> MSDTWSSIQAHKKQLDSLRERLQRRRKQDSGHLDLRNPEAALSPTFRSDSPVPTAPTSGGPKPSTASAVPELATDPELEKKLLHHLSDLALTLPTDAVSICLAISTPDAPATQDGVESLLQKFAAQELIEVKRGLLQDDAHPTLVTYADHSKLSAMMGAVAEKKGPGEVAGTVTGQKRRAEQDSTTVAAFASSLVSGLNSSASEPAKEPAKKSRKHAASDVDLEIESLLNQQSTKEQQSKKVSQEILELLNTTTAKEQSIVEKFRSRGRAQVQEFCDYGTKEECMKASDADRPCRKLHFRRIINKHTDESLGDCSFLNTCFHMDTCKYVHYEI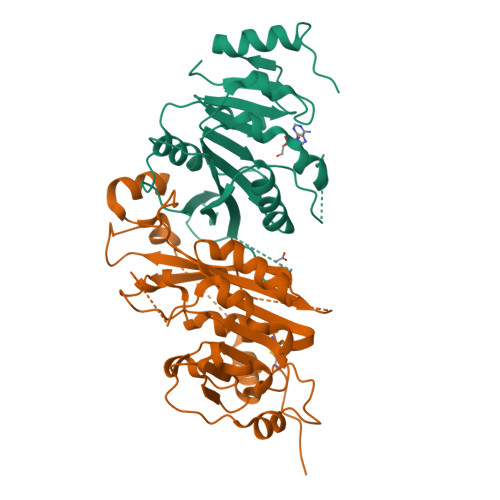DACMDSEAPGSKDHTPSQELALTQSVGGDSSADRLFPPQWICCDIRYLDVSILGKFAVVMADPPWDIHMELPYGTLTDDEMRRLNIPVLQDDGFLFLWVTGRAMELGRECLNLWGYERVDEIIWVKTNQLQRIIRTGRTGHWLNHGKEHCLVGVKGNPQGFNQGLDCDVIVAEVRSTSHKPDEIYGMIERLSPGTRKIELFGRPHNVQPNWITLGNQLDGIHLLDPDVVARFKQRYPDGIISKPKNL;> MDSRLQEIRERQKLRRQLLAQQLGAESADSIGAVLNSKDEQREIAETRETCRASYDTSAPNAKRKYLDEGETDEDKMEEYKDELEMQQDEENLPYEEEIYKDSSTFLKGTQSLNPHNDYCQHFVDTGHRPQNFIRDVGLADRFEEYPKLRELIRLKDELIAKSNTPPMYLQADIEAFDIRELTPKFDVILLEPPLEEYYRETGITANEKCWTWDDIMKLEIDEIAAPRSFIFLWCGSGEGLDLGRVCLRKWGYRRCEDICWIKTNKNNPGKTKTLDPKAVFQRTKEHCLMGIKGTVKRSTDGDFIHANVDIDLIITEEPEIGNIEKPVEIFHIIEHFCLGRRRLHLFGRDSTIRPGWLTVGPTLTNSNYNAETYASYFSAPNSYLTGCTEEIERLRPKSPPPKSKSDRGGGAPRGGGRGGTSAGRGRERNRSNFRGERGGFRGGRGGAHRGGFPPR>[6x]MDPIKQEISEYFKDWMELYKKNAIDEMTYKGYEQTLKYLKTYMP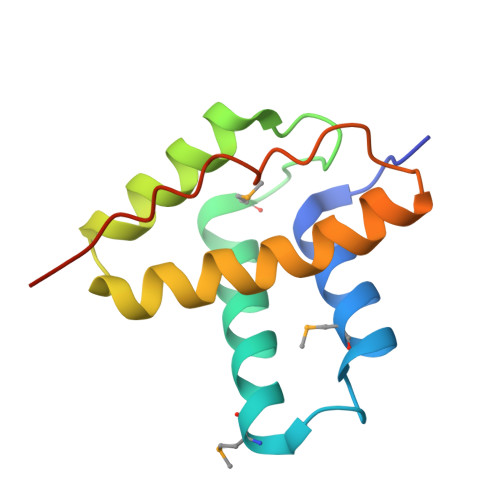NVLISEITASSYQRALNKFAETHAKASTKGFHTRVRASIQCLIEEGRLQKDFTTRAVVKGLEHHHHHH> TAEVMSHVTAHFGKTLEECREESGLSVDILDEF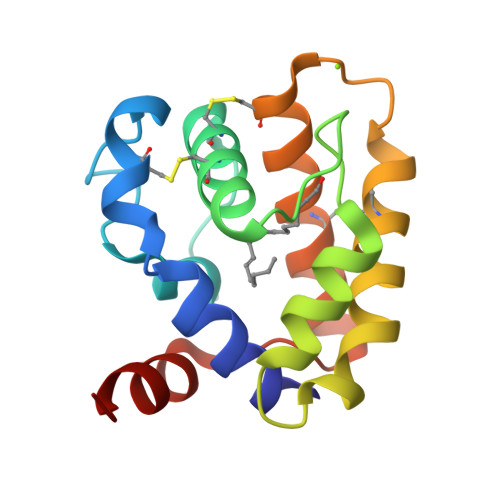KHFWSDDFDVVHRELGCAIICMSNKFSLMDDDVRMHHVNMDEYIKSFPNGQVLAEKMVKLIHNCEKQFDTETDDCTRVVKVAACFKEDSRKEGIAPEVAMVEAVIEKY> SADGCTDWSIDIKKYQVLVGEPVRIKCALFYGYIRTNYSLAQSAGLSLMWYKSSGPGDFEEPIAFDGSRMSKEEDSIWFRPTLLQDSGLYACVIRNSTYCMKVSISLTVGENDTGLCYNSKMKYFEKAELSKSKEISCRDIEDFLLPTREPEILWYKECRTKTWRPSIVFKRDTLLIREVREDDIGNYTCELKYGGFVVRRTTELTVTAPLTDKPPKLLYPMESKLTIQETQLGDSANL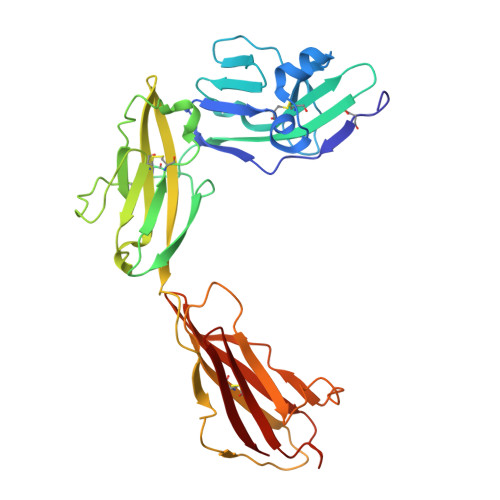TCRAFFGYSGDVSPLIYWMKGEKFIEDLDENRVWESDIRILKEHLGEQEVSISLIVDSVEEGDLGNYSCYVENGNGRRHASVLL>[2x]GSHMMPQLQFKDAFWCRDFTAHTGYEVLLQRLLDGRKMCKDMEELLRQRAQAEE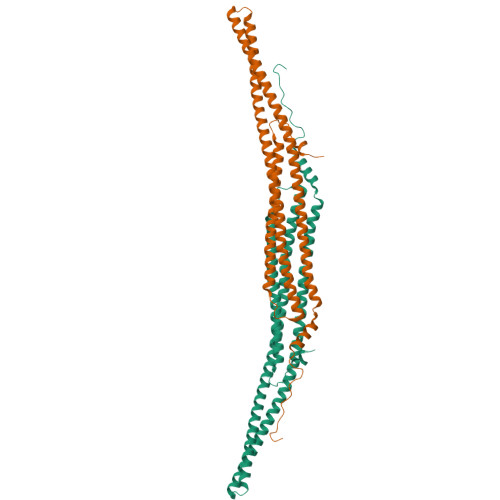RYGKELVQIARKAGGQTEINSLRASFDSLKQQMENVGSSHIQLALTLREELRSLEEFRERQKEQRKKYEAVMDRVQKSKLSLYKKAMESKKTYEQKCRDADDAEQAFERISANGHQKQVEKSQNKARQCKDSATEAERVYRQSIAQLEKVRAEWEQEHRTTCEAFQLQEFDRLTILRNALWVHSNQLSMQCVKDDELYEEVRLTLEGCSIDADIDSFIQAKSTGTEPPAPVPYQNYYD>ASLRANDAPIVLLHGFTGWGREEMFGFKYWGGVRGDIEQWLNDNGYRTYTLAVGPLSSNWDRVCEAYVQLVGGTVDYGAAHAAKHGHARFGRTYPGLLPELKRGGRIHIIA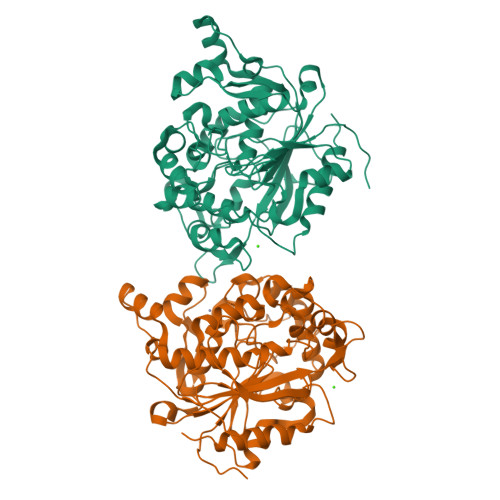HSQGGQTARMLVSLLENGSQEEREYAKAHNVSLSPLFEGGHHFVLSVTTIATPHDGTTLVNMVDFTDRFFDLQKAVLEAAAVASNVPYTSQVYDFKLDQWGLRRQPGESFDHYFERLKRSPVWTSTDTARYDLSVSGAEKLNQWVQASPNTYYLSFSTERTYRGALTGNHYPELGMNAFSAVVCAPFLGSYRNPTLGIDSHWLENDGIVNTISMNGPKRGSNDRIVPYDGTLKKGVWNDMGTYNVDHLEIIGVDPNPSFDIRAFYLRLAEQLASLQP[2x]Among them, the α1-adrenoceptor (α1AR) comprises 3 subtypes: α1AAR, α1BAR, and α1DAR, which mediate signal transduction via the activation of Gq/11 proteins. Antagonists targeting α1AR have been primarily utilized clinically for management of hypertension and benign prostatic hyperplasia (BPH). In this study, we determined the structures of α1AAR in complex with the α1AR-selective antagonist doxazosin and the α1AAR subtype–selective antagonist silodosin. The complex structures indicate that both doxazosin and silodosin bind to the orthosteric binding site of α1AAR.

Doxazosin is a selective α1AR antagonist that belongs to the quinazoline class of drugs. The structure of the doxazosin–α1AAR complex reveals that doxazosin adopts an inverted L-shaped conformation within the binding pocket of α1AAR, establishing extensive interactions with surrounding residues. Specifically, the dimethoxyquinazoline moiety of doxazosin inserts into the orthosteric site of α1AAR, forming hydrophobic contacts with multiple residues, including C1103.36, V1073.33, T1113.37, F2886.51, F2896.52, I1785.52, M2926.55, and Y1845.38. In addition to hydrophobic interactions, 3 key hydrogen bonds are observed: the oxygen atom of the dimethoxy group forms a hydrogen bond with S1885.42; the nitrogen atom in the pyrimidine ring forms a hydrogen bond with D1063.32; and the nitrogen atom in the amine group forms a hydrogen bond with Y1845.38. The other 2 moieties of doxazosin, the 1,4-benzodioxane-2-carbonyl and piperazine groups, are accommodated by α1AAR residues D1063.32, W1023.28, A1033.29, C17645.50, Q17745.51, F3127.39, K3097.36, F3087.35, Y3167.43, and F862.64, which are primarily located in TM2, TM3, and TM7. In contrast, doxazosin, with its more rigid quinazoline ring, appears to have a suboptimal fit in the pocket, resulting in its positioning more toward the receptor's outer region. Consequently, doxazosin fails to establish the π–π interactions with F2896.52, which are observed for silodosin and tamsulosin. In addition, van der Waals interactions involving residue E872.65 were observed only for silodosin and tamsulosin but absent in doxazosin-bound complex. Conversely, the inhibitory activity of doxazosin was not diminished by these substitutions, highlighting the crucial role of M2926.55 in determining ligand selectivity.

> APVNISKAILLGVILGGLILFGVLGNILVILSVACHRHLHSVTHYYIVNLAVADLLLTSTVLPFSAIFEVLGYWAFGRVFCNIWAAVDVLCCTASIMGLCIISIDRYIGVSYPLRYPTIVTQRRGLMALLCVWALSLVISIGPLFGWRQPAPEDETICQINEEPGYVLFSALGSFYLPLAIILVMYCRVYVVAKRESRGLKSGLKTDKSDSEQVTLRIHRKNAPAGGSGMASAKTKTHFSVRLLKFSREKKAAKTLGIVVGCFVLCWLPFFLVMPIGSFFPDFKPSETVFKIVFWLGYLNSCINPIIYPCSSQEFKKAFQNVL>[6x]MAAPARDPPGYRYAAAILPTGSILSTIEVASHRRLFDFFAAVRSDENSLYDVEFDALLGSYCNTLSLVRFLELGLSVACVCTKFPELAYMNEGRVQFEVHQPLIARDGPHPVEQPVHNYMTKVIDRRALNAAFSLATEAIALLTGEALDGTGISLHRQLRAIQQLARNVQAVLGAFERGTADQMLHVLLEKAPPLALLLPMQRYLDNGRLATRVARATLVAELKRSFCDTSFFLGKAGHRREAIEAWLVDLTTATQPSVAVPRLTHADTRGRPVDGVLVTTAAIKQRLLQSFLKVEDTEADVPVTYGEMVLNGANLVTALVMGKAVRSLDDVGRHLLDMQEEQLEANRETLDELESAPQTTRVRADLVAIGDRLVFLEALERRIYAATNVPYPLVGAMDLTFVLPLGLFNPAMERFAAHAGDLVPAPGHPEPRAFPPRQLFFWGKDHQVLRLSMENAVGTVCHPSLMNIDAAVGGVNHDPVEAANPYGAYVAAPAGPGADMQQRFLNAWRQRLAHGRVRWVAECQMTAEQFMQPDNANLALELHPAFDFFAGVADVELPGGEVPPAGPGAIQATWRVVNGNLPLALCPVAFRDARGLELGVGRHAMAPATIAAVRGAFEDRSYPAVFYLLQAAIHGNEHVFCALARLVTQCITSYWNNTRCAAFVNDYSLVSYIVTYLGGDLPEECMAVYRDLVAHVEALAQLVDDFTLPGPELGGQAQAELNHLMRDPALLPPLVWDCDGLMRHAALDRHRDCRIDAGGHEPVYAAACNVATADFNRNDGRLLHNTQARAADAADDRPHRPADWTVHHKIYYYVLVPAFSRGRCCTAGVRFDRVYATLQNMVVPEIAPGEECPSDPVTDPAHPLHPANLVANTVKRMFHNGRVVVDGPAMLTLQVLAHNMAERTTALLCSAAPDAGANTASTANMRIFDGALHAGVLLMAPQHLDHTIQNGEYFYVLPVHALFAGADHVANAPNFPPALRDLARDVPLVPPALGANYFSSIRQPVVQHARESAAGENALTYALMAGYFKMSPVALYHQLKTGLHPGFGFTVVRQDRFVTENVLFSERASEAYFLGQLQVARHETGGGVNFTLTQPRGNVDLGVGYTAVAATGTVRNPVTDMGNLPQNFYLGRGAPPLLDNAAAVYLRNAVVAGNRLGPAQPLPVFGCAQVPRRAGMDHGQDAVCEFIATPVATDINYFRRPCNPRGRAAGGVYAGDKEGDVIALMYDHGQSDPARPFAATANPWASQRFSYGDLLYNGAYHLNGASPVLSPCFKFFTAADITAKHRCLERLIVETGSAVSTATAASDVQFKRPPGCRELVEDPCGLFQEAYPITCASDPALLRSARDGEAHARETHFTQYLIYDASPLKGLSL;> MNAHFANEVQYDLTRDPSSPASLIHVIISSECLAAAGVPLSALMRGRPDGGAAANFRVETQTRAHATGDCTPWRSAFAAYVPADAVGALIAPVVPAHPDLLPRVPSAGGLFVSLPVACDAQGVYDPYTVAALRLAWGPWATCARVLLFSYDELVPPNTRYAADGARLMRLCRHFCRYVARLGAAAPAAATEAAAHLSMGLGESGTPTPQASSVSGGAGPAVVGTPDPPISPEEQLTAPGGDTATAEDVSITQENEEILALVQRAVQDVTRRHPVRARPKHAASGVASGLRQGALVHQAVSGGALGASDAEAVLAGLEPPGGGRFASRGGPRAAGEDVLNDVLTLVPGTAKPRSLVEWLDRGWEALAGGDRPDWLWSRRSISVVLRHHYGTKQRFVVVSYENSVAWGGRRARPPRLSSELATALTEACAAERVVRPHQLSPAAQTALLRRFPALEGPLRHPRPVLQPFDIAAEVAFVARIQIACLRALGHSIRAALQGGPRIFQRLRYDFGPHQSEWLGEVTRRFPVLLENLMRALEGTAPDAFFHTAYALAVLAHLGGQGGRGRRRRLVPLSDDIPARFADSDAHYAFDYYSTSGDTLRLTNRPIAVVIDGDVNGREQSKCRFMEGSPSTAPHRVCEQYLPGESYAYLCLGFNRRLCGLVVFPGGFAFTINTAAYLSLADPVARAVGLRFCRGAATGPGLVR;>MDPYYPFDALDVWEHRRFIVADSRSFITPEFPRDFYMSPVFNIPRETAAERAAVLQAQRTAAAAALENAALQAAELPVDIERRIRPIEQQVHHIADALEALETAATAAEEADAARDAEARGEGAADGAAPSPTAGPAAAEMEVQIVRNDPPLRYDTNLPVDLLHMVYAGRGAAGSSGVVFGTWYRTIQERTIADFPLTTRSADFRDGRMSKTFMTALVLSLQSCGRLYVGQRHYSAFECAVLCLYLLYRTTHESSPDRDRAPVAFGDLLARLPRYLARLAAVIGDESGRPQYRYRDDKLPKAQFAAAGGRYEHGALATHVVIATLVRHGVLPAAPGDVPRDTSTRVNPDDVAHRDDVNRAAAAFLARGHNLFLWEDQTLLRATANTITALAVLRRLLANGNVYADRLDNRLQLGMLIPGAVPAEAIARGASGLDSGAIKSGDNNLEALCVNYVLPLYQADPTVELTQLFPGLAALCLDAQAGRPLASTRRVVDMSSGARQAALVRLTALELINRTRTNTTPVGEIINAHDALGIQYEQGLGLLAQQARIGLASNAKRFATFNVGSDYDLLYFLCLGFIPQYLSVA[2x];>MAAPQFHRPSTIT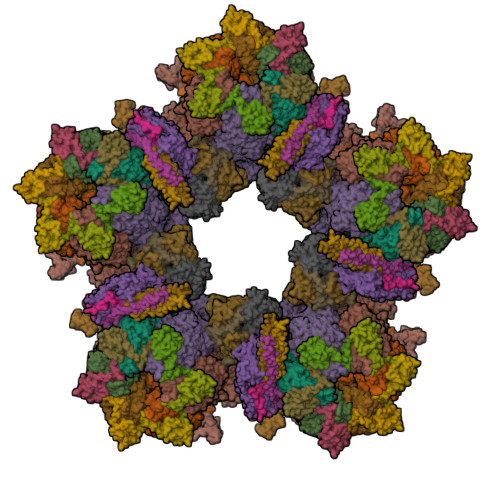ADNVRALGMRGLVLATNNAQFIMDNSYPHPHGTQGAVREFLRGQAAALTDLGVTHANNTFAPQPMFAGDAAAEWLRPSFGLKRTYSPFVVRDPKTPSTP[6x];>MIPAALPHPTMKRQGDRDIVVTGVRNQFATDLEPGGSVSCMRSSLSFLSLLFDVGPRDVLSAEAIEGCLVEGGEWTRAAAGSGPPRMCSIIELPNFLEYPAARGGLRCVFSRVYGEVGFFGEPTAGLLETQCPAHTFFAGPWAMRPLSYTLLTIGPLGMGLYRDGDTAYLFDPHGLPAGTPAFIAKVRAGDVYPYLTYYAHDRPKVRWAGAMVFFVPSGPGAVAPADLTAAALHLYGASETYLQDEPFVERRVAITHPLRGEIGGLGALFVGVVPRGDGEGSGPVVPALPAPTHVQTPGADRPPEAPRGASGPPDTPQAGHPNRPPDDVWAAALEGTPPAKPSAPDAAASGPPHAAPPPQTPAGDAAEEAEDLRVLEVGAVPVGRHRARYSTGLPKRRRPTWTPPSSVEDLTSGERPAPKAPPAKAKKKSAPKKKAPVAAEVPASSPTPIAATVPPAPDTPPQSGQGGGDDGPASPSSPSVLETLGARRPPEPPGADLAQLFEVHPNVAATAVRLAARDAALAREVAACSQLTINALRSPYPAHPGLLELCVIFFFERVLAFLIENGARTHTQAGVAGPAAALLDFTLRMLPRKTAVGDFLASTRMSLADVAAHRPLIQHVLDENSQIGRLALAKLVLVARDVIRETDAFYGDLADLDLQLRAAPPANLYARLGEWLLERSRAHPNTLFAPATPTHPEPLLHRIQALAQFARGEEMRVEAEAREMREALDALARGVDSVSQRAGPLTVMPVPAAPGAGGRAPCPPALGPEAIQARLEDVRIQARRAIESAVKEYFHRGAVYSAKALQASDSHDCRFHVASAAVVPMVQLLESLPAFDQHTRDVAQRAALPPPPPLATSPQAILLRDLLQRGQPLDAPEDLAAWLSVLTDAATQGLIERKPLEELARSIHGINDQQARRSSGLAELQRFDALDAALAQQLDSDAAFVPATGPAPYVDGGGLSPEATRMAEDALRQARAMEAAKMTAELAPEARSRLRERAHALEAMLNDARERAKVAHDAREKFLHKLQGVLRPLPDFVGLKACPAVLATLRASLPAGWTDLADAVRGPPPEVTAALRADLWGLLGQYREALEHPTPDTATALAGLHPAFVVVLKTLFADAPETPVLVQFFSDHAPTIAKAVSNAINAGSAAVATASPAATVDAAVRAHGALADAVSALGAAARDPASPLSFLAVLADSAAGYVKATRLALEARGAIDELTTLGSAAADLVVQARRACAQPEGDHAALIDAAARATTAARESLAGHEAGFGGLLHAEGTAGDHSPSGRALQELGKVIGATRRRADELEAAVADLTAKMAAQRARGSSERWAAGVEAALDRVENRAEFDVVELRRLQALAGTHGYNPRDFRKRAEQALAANAEAVTLALDTAFAFNPYTPENQRHPMLPPLAAIHRLGWSAAFHAAAETYADMFRVDAEPLARLLRIAEGLLEMAQAGDGFIDYHEAVGRLADDMTSVPGLRRYVPFFQHGYADYVELRDRLDAIRADVHRALGGVPLDLAAAAEQISAARNDPEATAELVRTGVTLPCPSEDALVACAAALERVDQSPVKNTAYAEYVAFVTRQDTAETKDAVVRAKQQRAEATERVMAGLREALAARERRAQIEAEGLANLKTMLKVVAVPATVAKTLDQARSVAEIADQVEVLLDQTEKTRELDVPAVIWLEHAQRTFETHPLSAARGDGPGPLARHAGRLGALFDTRRRVDALRRSLEEAEAEWDEVWGRFGRVRGGAWKSPEGFRAMHEQLRALQDTTNTVSGLRAQPAYERLSARYQGVLGAKGAERAEAVEELGARVTKHTALCARLRDEVVRRVPWEMNFDALGGLLAEFDAAAADLAPWAVEEFRGARELIQYRMGLYSAYARAGGQTGAGAESAPAPLLVDLRALDARARASSSPEGHEVDPQLLRRRGEAYLRAGGDPGPLVLREAVSALDLPFATSFLAPDGTPLQYALCFPAVTDKLGALLMRPEAACVRPPLPTDVLESAPTVTAMYVLTVVNRLQLALSDAQAANFQLFGRFVRHRQATWGASMDAAAELYVALVATTLTREFGCRWAQLGWASGAAAPRPPPGPRGSQRHCVAFNENDVLVALVAGVPEHIYNFWRLDLVRQHEYMHLTLERAFEDAAESMLFVQRLTPHPDARIRVLPTFLDGGPPTRGLLFGTRLADWRRGKLSETDPLAPWRSALELGTQRRDVPALGKLSPAQALAAVSVLGRMCLPSAALAALWTCMFPDDYTEYDSFDALLAARLESGQTLGPAGGREASLPEAPHALYRPTGQHVAVLAAATHRTPAARVTAMDLVLAAVLLGAPVVVALRNTTAFSRESELELCLTLFDSRPGGPDAALRDVVSSDIETWAVGLLHTDLNPIENACLAAQLPRLSALIAERPLADGPPCLVLVDISMTPVAVLWEAPEPPGPPDVRFVGSEATEELPFVATAGDVLAASAADADPFFARAILGRPFDASLLTGELFPGHPVYQRPLADEAGPSAPTAARDPRDLAGGDGGSGPEDPAAPPARQADPGVLAPTLLTDATTGEPVPPRMWAWIHGLEELASDDAGGPTPNPAPALLPPPATDQSVPTSQYAPRPIGPAATARETRPSVPPQQNTGRVPVAPRDDPRPSPPTPSPPADAALPPPAFSGSAAAFSAAVPRVRRSRRTRAKSRAPRASAPPEGWRPPALPAPVAPVAASARPPDQPPTPESAPPAWVSALPLPPGPASARGAFPAPTLAPIPPPPAEGAVVPGGDRRRGRRQTTAGPSPTPPRGPAAGPPRRLTRPAVASLSASLNSLPSPRDPADHAAAVSAAAAAVPPSPGLAPPTSAVQTSPPPLAPGPVAPSEPLCGWVVPGGPVARRPPPQSPATKPAARTRIRARSVPQPPLPQPPLPQPPLPQPPLPQPPLPQPPLPQPPLPQPPLPQPPLPQPPLPQPPLPPVTRTLTPQSRDSVPTPESPTHTNTHLPVSAVTSWASSLALHVDSAPPPASLLQTLHISSDDEHSDADSLRFSDSDDTEALDPLPPEPHLPPADEPPGPLAADHLQSPHSQFGPLPVQANAVLSRRYVRRTGRSALAVLIRACRRIQQQLQRTRRALFQRSNAVLTSLHHVRMLLG[2x];>[2x]MITDCFEADIAIPSGISRPDAAALQRCEGRVVFLPTIRRQLALADVAHESFVSGGVSPDTLGLLLAYRRRFPAVITRVLPTRIVACPVDLGLTHAGTVNLRNTSPVDLCNGDPVSLVPPVFEGQATDVRLESLDLTLRFPVPLPTPLAREIVARLVARGIRDLNPDPRTPGELPDLNVLYYNGARLSLVADVQQLASVNTELRSLVLNMVYSITEGTTLILTLIPRLLALSAQDGYVNALLQMQSVTREAAQLIHPEAPMLMQDGERRLPLYEALVAWLAHAGQLGDILALAPAVRVCTFDGAAVVQSGDMAPVIRYP;> MKTKPLPTAPMAWAESAVETTTSPRELAGHAPLRRVLRPPIARRDGPVLLGDRAPRRTASTMWLLGIDPAESSPGTRATRDDTEQAVDKILRGARRAGGLTVPGAPRYHLTRQVTLTDLCQPNAERAGALLLALRHPTDLPHLARHRAPPGRQTERLAEAWGQLLEASALGSGRAESGCARAGLVSFNFLVAACAAAYDARDAAEAVRAHITTNYGGTRAGARLDRFSECLRAMVHTHVFPHEVMRFFGGLVSWVTQDELASVTAVCSGPQEATHTGHPGRPCSAVTIPACAFVDLDAELCLGGPGAAFLYLVFTYRQCRDQELCCVYVVKSQLPPRGLEAALERLFGRLRITNTIHGAEDMTPPPPNRNVDFPLAVLAASSQSPRCSASQVTNPQFVDRLYRWQPDLRGRPTARTCTYAAFAELGVMPDDSPRCLHRTERFGAVGVPVVILEGVVWRPGGWRACA>MATTIKENEFLCDEEIYKSFVHLKDKICEERKKKELVSYSSYIKEMKKLLKVVLLKYKALKFGEFILKSKRKSNYFFSSGVLNNIVSSNIIC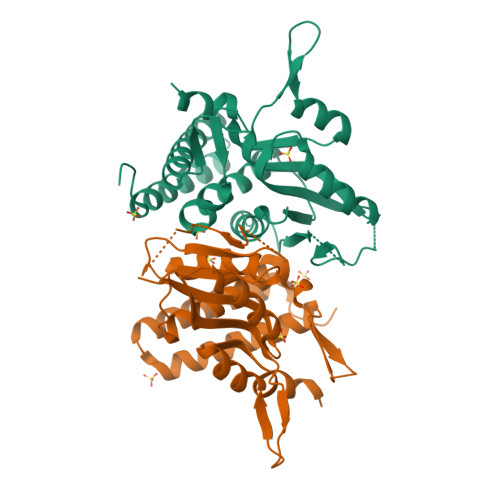FLLSELILKNKLSFDYLLGASYKGIPMVSLTSHFLFESKKYSNIFYLYDRKEKKEYGDKNVIVGNLDDDDKDILNLKKKTKNNQDEEKKNIIIIDDVFTCGTALTEILAKLKTYEHLKVVAFIVLLNRNEYEINENNQKIYFKDIFEKRVGIPLYSILSYKDDIQSMIHHHHHH[8x]4-({[(4-fluorophenyl)methyl]amino}methyl)benzonitrile 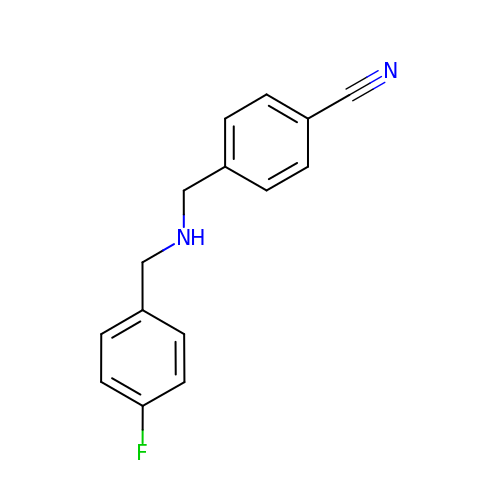| C15 H13 F N2 | DLXXWXOFLPDGAD-UHFFFAOYSA-N~{N}-(2-chloranyl-6-methyl-phenyl)-2-[(3,5-dimorpholin-4-ylphenyl)amino]-1,3-thiazole-5-carboxamide | 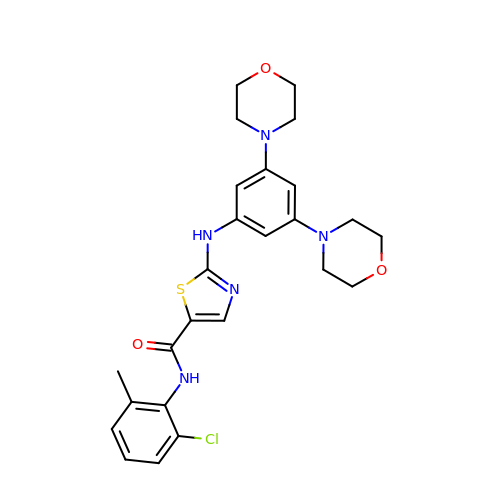C25 H28 Cl N5 O3 S | FISCIEKUXURIRB-UHFFFAOYSA-N>[2x]DHYNCVSS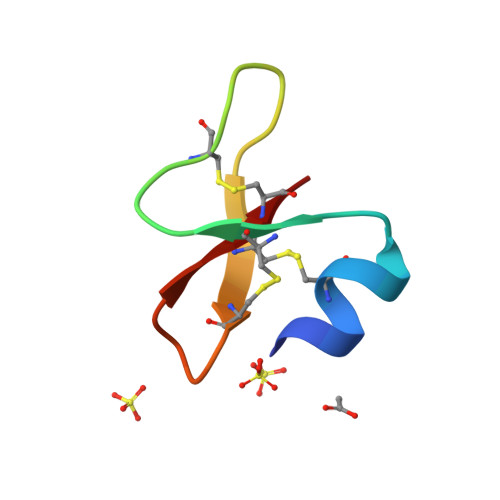GGQCAYSACPIFTKIQGTCYRGKAKCCK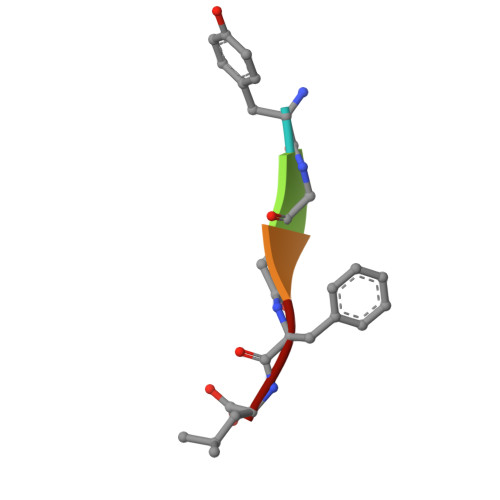> YGGFL> GGNRTFSYTLEDHTKQAAGIMNELRLSQQLCDVTLQVKYQDAPAAQFMAHKVVLA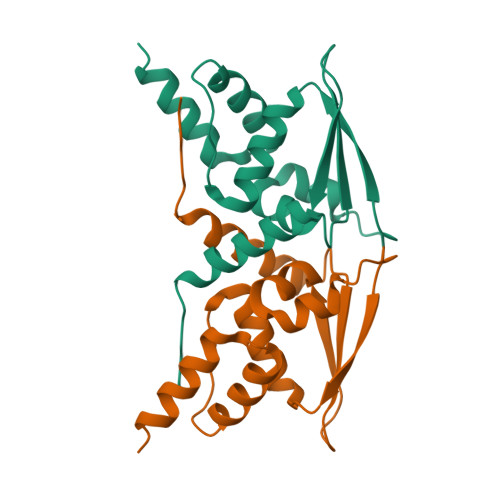SSSPVFKAMFTNGLREQGMEVVSIEGIHPKVMERLIEFAYTASISMGEKCVLHVMNGAVMYQIDSVVRACADFLVQQLD> YANATS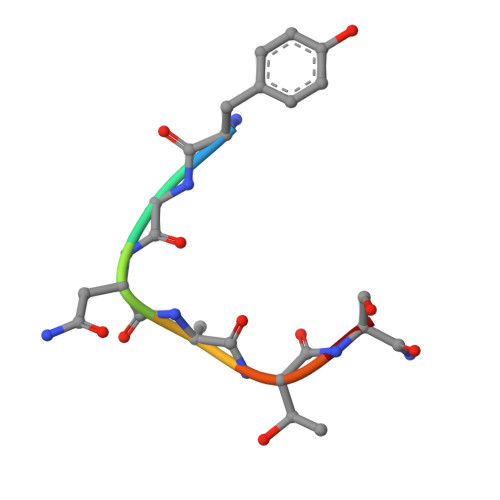A> GRNQKPSRLTRSANNVLLEKGPTVERSTRMSNPWKAFMEKYDIERTHSSGVRVDLGEDAEVENAKYRIPAGRCPVFGKGIVIENSAVSFLKPVATGDQRLKDGGFAFPNANDHISPMTLENLKARYKDNVEMMKLNDIALCRTHAASFVMAGDQNSNYRHPAVYDEKEKTCHMLYLSAQENMGPRYCSPDAQNRDAVFCFKPDKDESFENLVYLSKNVRNDWDKKCPRKNLGNAKFGLWVDGNCEEIPYVKEVEAKDLRECNRIVFEASASDQPTQYEEEMTDYQKIQQGFRQNNREMIKSAFLPVGAFNSDNFKSKGRGFNWANFDSVKKKCYIFNTKPTCLINDKNFIATTALSHPREVDLEFPCSIYKDEIEREIKKQSRNMNLYSVDGERIVLPRIFISNDKESIKCPCEPEHISQSTCNFYVCNCVEKRAEIKENNQVVIKEEFRDYYENGEEKSNK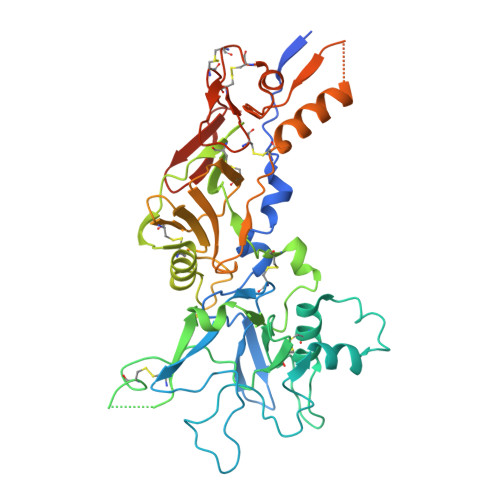QGS>[2x]MENSNNKRAPYWTNTEKMEKRLHAVPAANTVKFRCPAGGNPMPT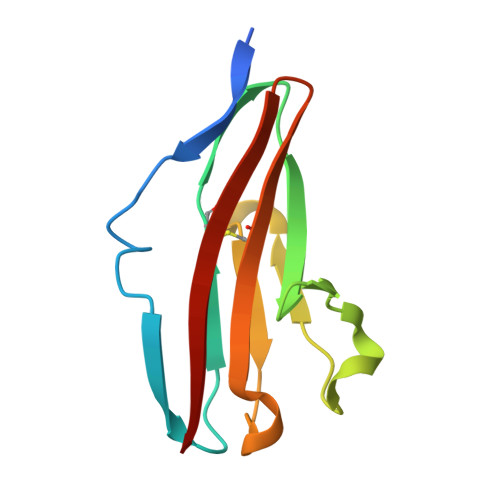MRWLKNGKEFKQEHRIGGYKVRNQHWSLIMESVVPSDKGNYTCVVENEYGSINHTYHLDVV>GSVTALSDVNNTDNYGAGQIQVLEGLEAVRKRPGMYIGSTSERGLHHLVWEIVDNSIDEALAGYANQIEVVIEKDNWIKVTDNGRGIPVDIQEKMGRPAVEVILTSSVVNALSQDLEVYVHRNETIYHQAYKKGVPQFDLKEVGTTDKTGTVIR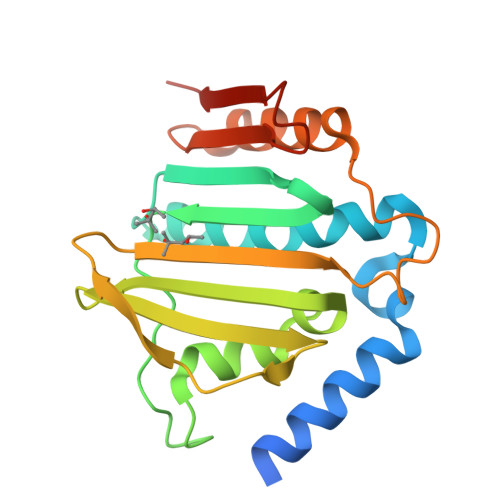FKADGEIFTETTVYNYETLQQRIRELAFLNKGIQITLRDERDEENVREDSYHYEGGIK[2x]>GHMMTLPESKDFSYLFSDETNARKPSPLKTCIHLFQDPNIIFLGGGLPLKDYFPWDNLSVDSPKPPFPQGIGAPIDEQNCIKYTVNKDYADKSANPSNDIPLSRALQYGFSAGQPELLNFIRDHTKIIHDLKYKDWDVLATAGNTNAWESTLRVFCNRGDVILVEAHSFSSSLASAEAQGVITFPVPIDADGIIPEKLAKVMENWTPGAPKPKLLYTIPTGQNPTGTSIADHRKEAIYKIAQKYDFLIVEDEPYYFLQMNPYIKDLKEREKAQSSPKQDHDEFLKSLANTFLSLDTEGRVIRMDSFSKVLAPGTRLGWITGSSKILKPYLSLHEMTIQAPAGFTQVLVNATLSRWGQKGYLDWLLGLRHEYTLKRDCAIDALYKYLPQSDAFVINPPIAGMFFT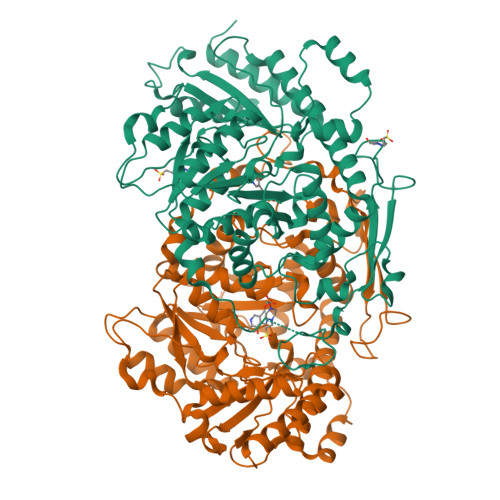VNIDASVHPEFKTKYNSDPYQLEQSLYHKVVERGVLVVPGSWFKSEGETEPPQPAESKEVSNPNIIFFRGTYAAVSPEKLTEGLKRLGDTLYEEFGISK[4x]> AMADIGSDKCKKTTTCEP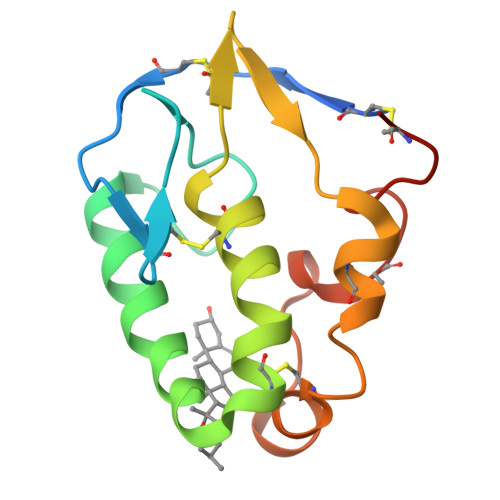LKYNICLGSVLPYALTSTVLAEDSSSQDEVHDKLSLWSGLRNAPRCWDAIRPLLCAVYMPKCEGGKVELPSQGLCQTTRVPCAIVARERGWPDFLKCTTDYFPEGCPNE> MSKVMKPSNGKGSRKSSKAATPDTKNFFHAKKKDPVNQDKANNASQITPTVPHSHPSDMVIPDHLAELIPELYSFQQLVDSEKRLDHFIHLRNLHMKRMVAQWERSKLSQEFLYPHLNFPNVKFLRIFISNVSENQPWQMDTNNEADLMALENATWTMRIEGRLLDNVQANDPAREKFSSFIESIVVDFKNKENDNVPSTKFNAAPEENATEGPSDKKLNLNLPLQFSLPNGDNSTTTNTDQNNATMGEETAKKDMSSTTPKLESVKWQYDPNNPVDFDGLDIKRVGSENVECTISILRKSSPEEPFMSYSPQLTAIIGLKSGTSHDAIFSIYKYIHLNELLTNDESAFENLMGNRNNHNSNTSTSKMLDAASSQVSIVKLDTQLITLLPSSLKESSPDTMKLTDLLSLINSTHLLPLQPIEIDYTVRVDKASTYGELVLDIEVPDVNALKFNNTQRESQIGAAELNENARELEQIKPKIALQDKEITSVLSNLHESNKRYRFFKKISEDPVKALNECIASTSNALKVLSGDEGYNEDMVRRANFYKENEAMLRENIEVILSNGRM;>MENTLGEGSTVNASVDVDQHGNDNNSDSNANAAVAGVANTDTAGEESQQQDESLKDEATVPNTRDAESEAITVTAKQQPTMQANKLDSQETPSTEESRAQNVFGQDNEDSDNLFGETESSVSNNEANTPSIPTNPVDNENNKPAIKEDSTIQDSNGDVKNMEDVKIQKEEEPENNTVIEGVKEESQPDENTKEMDEVEEDDEDDDQPMISPDNSIFGDTKSESKQLGNTSSVANTPSEIPDAHKAEQEDIIEKTESVDKKVDSGEERNEQEREIMNDHSKSANPKKTTITRVEPETFEIPQAHEIVIPSYSKWFNLEKIHSIEVQSLPEFFTNRIPSKTPEVYMRYRNFMVNSYRLNPNEYFSVTTARRNVSGDAAALFRLHKFLTKWGLINYQVDSKLLPKNIEPPLTSQYSTRHDAPRGLFPFESYKPSVQLPDMAKLKKMMNTSDSESTLYKYLKESKRKYDEITHPPSTTDDENGDKNDNGGKMNNEVSTSTSMTGDANLLEEGETSRPLKKVKILEQIDENWSKEDLQKLLKGIQEFGADWYKVAKNVGNKSPEQCILRFLQLPIEDKFLYGDGNGKGDNDNGLGPLKYAPHLPFSKSENPVLSTIAFLVGLVNPKTVQSMTQRAIQSAESIKSQKEEISDQKPIEHIKEGSEIAISSLGYRSHIFATNEERQMNFLTNELIRLQMEKLDAKLNHLKKLEKFMELERKTLERQQENLLIQRLNFNQNSSKIVNVLSKCLNLISDSNINNSSVAEKEEIRSQIDHFKSMLSKPETLSIGKNPFNKPNIETGENHNGQSISNENDVKPISIEAPQFYRYWSA[2x];> MGVIKKKRSHHGKASRQQYYSGVQVGGVGSMGAINNNIPSLTSFAEENNYQYGYSGSSAGMNGRSLTYAQQQLNKQRQDFERVRLRPEQLSNIIHDESDTISFRSNLLKNFISSNDAFNMLSLTTVPCDRIEKSRLFSEKTIRYLMQKQHEMKTQAAELQEKPLTPLKYTKLIAAAEDGSRSTKDMIDAVFEQDSHLRYQPDGVVVHRDDPALVGKLRGDLREAPADYWTHAYRDVLAQYHEAKERIRQKEVTAGEAQDEASLQQQQQQDLQQQQQVVTTVASQSPHATATEKEPVPAVVDDPLENMFGDYSNEPFNTNFDDEFGDLDAVFF;> MLGEDEGNTVLEKGNNPSVKQGEVGAVFIVPKILIREHERVILKQILQILDQDELVQPPLDKFPYKKLELPKYIDELKTRDATNTSYKMIQLDAYGEKKVGSNGELFGGRHYLFNTFTFTAHMGVLLVLLQDVIKVLYQSNATHDEDEFIVQHDQILVMETSEEQTKFLAKNGVIPEESKGSFKYITARSAFVEFGASVIAGGQRIVDDYWESLAKKQNLSSHQRVFKLSTNLISKISLLRPSFQNNRISNANEISANTNNTCTISTSKFESQYPIVTEQPSAEIREAYIENFAKGEHISAIVPGQSISGTLELSAQFRVPRYHSKNSFQQALQMKAMDIPIGRHEELLAQYESQAPDGSASISLPNHIPSVNPSNKPIKRMLSSILDINVSSSKNKKSEENEMIKPMNKGQHKNNTSLNINGWKFESLPLKSAENSGKQQYYRGLPLYEKNTLLERLKQLTPNEIKELEHLHDAVFVNTGLQNVRKVRTKKWKKYWQYKAGIPIGLKRSQLDEFKNKYLKDVLAQTSVTTNFNEITNTDETITTKRVPNPNFLGNCNIKDFKPPYIYSHVNKVPQNVAGDKTAVKLDTEVKNTNANPVVATDPVAAKPDNLANFSNEVAMNN;> MNNQPQGTNSVPNSIGNIFSNIGTPSFNMAQIPQQLYQSLTPQQLQMIQQRHQQLLRSRLQQQQQQQQQTSPPPQTHQSPPPPPQQSQPIANQSATSTPPPPPAPHNLHPQIGQVPLAPAPINLPPQIAQLPLATQQQVLNKLRQQAIAKNNPQVVNAITVAQQQVQRQIEQQKGQQTAQTQLEQQRQLLVQQQQQQQLRNQIQRQQQQQFRHHVQIQQQQQKQQQQQQQHQQQQQQQQQQQQQQQQQQQQQQQQQQQQQQQQQQQQQGQIPQSQQVPQVRSMSGQPPTNVQPTIGQLPQLPKLNLPKYQTIQYDPPETKLPYPTYWSDKKADTDTLLYEQIIQRDKINKYSLIRETNGYDPFSIYGFSNKEYISRLWHTLKYYQDLKNTRMKSITSTSQKIPSASIWGNGYSGYGNGITNTTTRVIPQVEVGNRKHYLEDKLKVYKQAMNETSEQLVPIRLEFDQDRDRFFLRDTLLWNKNDKLIKIEDFVDDMLRDYRFEDATREQHIDTICQSIQEQIQEFQGNPYIELNQDRLGGDDLRIRIKLDIVVGQNQLIDQFEWDISNSDNCPEEFAESMCQELELPGEFVTAIAHSIREQVHMYHKSLALLGYNFDGSAIEDDDIRSRMLPTITLDDVYRPAAESKIFTPNLLQISAAELERLDKDKDRDTRRKRRQGRSNRRGMLALSGTSASNTSMNGVHNTVAAGNASSLPPGEILLPDIADIPRTFRTPVPSTLMPGGVDVGPSVESYELRNTTTYKSRPDRPKPVSPPCYIIDHIPGHSLLLSIKLPGKVNTKEEFAAAPNDTSSGTNAMLPSPESLKTKLNSNIRAGVTIPSIPNPIANHTVTNSPNPTLQPVIPGGAASKSVPTPSLPIAPPVAPHDSEATLLTNSNNGSSNNNTQNT;> MNIPQRQFSNEEVNRCYLRWQHLRNEHGMNAPSVPEFIYLTKVLQFAAKQRQELQMQRQQQGISGSQQNIVPNSSDQAELPNNASSHISASASPHLAPNMQLNGNETFSTSAHQSPIMQTQMPLNSNGGNNMLPQRQSSVGSLNATNFSPTPANNGENAAEKPDNSNHNNLNLNNSELQPQNRSLQEHNIQDSNVMPGSQINSPMPQQAQMQQAQFQAQQAQQAQQAQQAQQAQARLQQGRRLPMTMFTAEQSELLKAQITSLKCLVNRKPIPFEFQAVIQKSINHPPDFKRMLLSLSEFARRRQPTDQNNQSNLNGGNNTQQPGTNSHYNNTNTDNVSGLTRNAPLDSKDENFASVSPAGPSSVHNAKNGTLDKNSQTVSGTPITQTESKKEENETISNVAKTAPNSNKTHTEQNNPPKPQKPVPLNVLQDQYKEGIKVVDIDDPDMMVDSFTMPNISHSNIDYQTLLANSDHAKFTIEPGVLPVGIDTHTATDIYQTLIALNLDTTVNDCLDKLLNDECTESTRENALYDYYALQLLPLQKAVRGHVLQFEWHQNSLLTNTHPNFLSKIRNINVQDALLTNQLYKNHELLKLERKKTEAVARLKSMNKSAINQYNRRQDKKNKRLKFGHRLIATHTNLERDEQKRAEKKAKERLQALKANDEEAYIKLLDQTKDTRITHLLRQTNAFLDSLTRAVKDQQKYTKEMIDSHIKEASEEVDDLSMVPKMKDEEYDDDDDNSNVDYYNVAHRIKEDIKKQPSILVGGTLKDYQIKGLQWMVSLFNNHLNGILADEMGLGKTIQTISLLTYLYEMKNIRGPYLVIVPLSTLSNWSSEFAKWAPTLRTISFKGSPNERKAKQAKIRAGEFDVVLTTFEYIIKERALLSKVKWVHMIIDEGHRMKNAQSKLSLTLNTHYHADYRLILTGTPLQNNLPELWALLNFVLPKIFNSVKSFDEWFNTPFANTGGQDKIELSEEETLLVIRRLHKVLRPFLLRRLKKDVEKELPDKVEKVVKCKMSALQQIMYQQMLKYRRLFIGDQNNKKMVGLRGFNNQIMQLKKICNHPFVFEEVEDQINPTRETNDDIWRVAGKFELLDRILPKLKATGHRVLIFFQMTQIMDIMEDFLRYINIKYLRLDGHTKSDERSELLRLFNAPDSEYLCFILSTRAGGLGLNLQTADTVIIFDTDWNPHQDLQAQDRAHRIGQKNEVRILRLITTNSVEEVILERAYKKLDIDGKVIQAGKFDNKSTSEEQEALLRSLLDAEEERRKKRESGVEEEEELKDSEINEILARNDEEMAVLTRMDEDRSKKEEELGVKSRLLEKSELPDIYSRDIGAELKREESESAAVYNGRGARERKTATYNDNMSEEQWLRQFEVSDDEKNDKQARKQRTKKEDKSEAIDGNGEIKGENIDADNDGPRINNISAEDRADTDLAMNDDDFLSKKRKAGRPRGRPKKVKLEGSENSEPPALESSPVTGDNSPSEDFMDIPKPRTAGKTSVKSARTSTRGRGRGRGRGRGRGRGRGRPPKARNGLDYVRTPAAATSPIDIREKVAKQALDLYHFALNYENEAGRKLSDIFLSKPSKALYPDYYMIIKYPVAFDNINTHIETLAYNSLKETLQDFH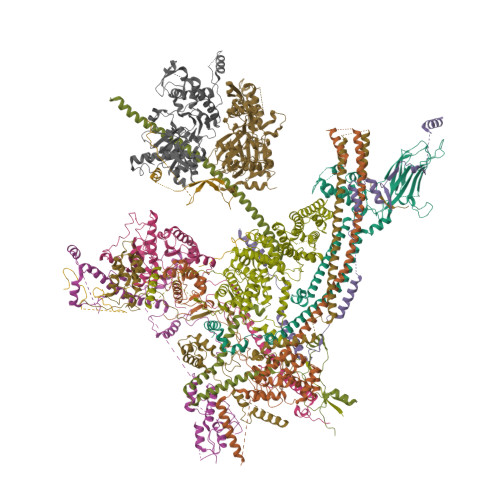LIFSNARIYNTEGSVVYEDSLELEKVVTKKYCEIMGDNSQLDFTEFDEQYGTRPLVLPPVVTSSVAESFTDEADSSMTEASV;> MDFFNLNNNNNNNNTTTTTTTTNNNNTNNNNTNNNNNPANNTNNNNSTGHSSNTNNNTNNNNTNTGASGVDDFQNFFDPKPFDQNLDSNNNNSNSNNNDNNNSNTVASSTNFTSPTAVVNNAAPANVTGGKAANFIQNQSPQFNSPYDSNNSNTNLNSLSPQAILAKNSIIDSSNLPLQAQQQLYGGNNNNNSTGIANDNVITPHFITNVQSISQNSSSSTPNTNSNSTPNANQQFLPFNNSASNNGNLTSNQLISNYAASNSMDRSSSASNEFVPNTSDNNNNSNNHNMRNNSNNKTSNNNNVTAVPAATPANTNNSTSNANTVFSERAAMFAALQQKQQQRFQALQQQQQQQQNQQQQNQQPQQQQQQQQNPKFLQSQRQQQQRSILQSLNPALQEKISTELNNKQYELFMKSLIENCKKRNMPLQSIPEIGNRKINLFYLYMLVQKFGGADQVTRTQQWSMVAQRLQISDYQQLESIYFRILLPYERHMISQEGIKETQAKRIFLQQFLQELLKKVQQQQQAAALANANNNINSASSAPTPAAPGASVPATAAPGTEAGIVPVSANTPKSLNSNININVNNNNIGQQQVKKPRKQRVKKKTKKELELERKEREDFQKRQQKLLEDQQRQQKLLLETKLRQQYEIELKKLPKVYKRSIVRNYKPLINRLKHYNGYDINYISKIGEKIDSNKPIFLFAPELGAINLHALSMSLQSKNLGEINTALNTLLVTSADSNLKISLVKYPELLDSLAILGMNLLSNLSQNVVPYHRNTSDYYYEDAGSNQYYVTQHDKMVDKIFEKVNNNATLTPNDSNDEKVTILVDSLTGNQLPTPTPTEMEPDLDTECFISMQSTSPAVKQWDLLPEPIRFLPNQFPLKIHRTPYLTSLKKIKDEIDDPFTKINTRGAEDPKVLINDQLSTISMILRNISFSDNNSRIMSRNFYLKRFISDLLWLVLIHPENFTCNRKILNFKKDLVIVLSNISHLLEIASSIDCLLILILVISFGQPKLNPMASSSSFGSESLTFNEFQLQWGKYQTFGVDILAKLFSLEKPNLNYFKSILLNKNTGNNLYDRNSNNNHKDKKLLRRLLNLYNDNNKNNNNRHNLLNDVVSFLFSAIPLQQVLSQSADPSLLIDQFSPVISQSLTSILVIVQKILPLSNEVFEISENNSDSNSNNNGNKDSSFNFNKNLPFVWLSSEENIGSGLLKLSEIILNINNSTSKNTLLQQQNYSKVLLPSINISCVQLIKCLVEKSICFENCLNNDPEILKKIASIPNLFPTDLEIFQLFTNPSVDIQIINQYQLLYNLKNDILTNLE;> MDPQTLITKANKVSYYGNPTSKESWRYDWYQPSKVSSNVQQPQQQLGDMENNLEKYPFRYKTWLRNQEDEKNLQRESCEDILDLKEFDRRILKKSLMTSHTKGDTSKATGAPSANQGDEALSVDDIRGAVGNSEAIPGLSAGVNNDNTKESKDVKMN;> MTLNRKCVVIHNGSHRTVAGFSNVELPQCIIPSSYIKRTDEGGEAEFIFGTYNMIDAAAEKRNGDEVYTLVDSQGLPYNWDALEMQWRYLYDTQLKVSPEELPLVITMPATNGKPDMAILERYYELAFDKLNVPVFQIVIEPLAIALSMGKSSAFVIDIGASGCNVTPIIDGIVVKNAVVRSKFGGDFLDFQVHERLAPLIKEENDMENMADEQKRSTDVWYEASTWIQQFKSTMLQVSEKDLFELERYYKEQADIYAKQQEQLKQMDQQLQYTALTGSPNNPLVQKKNFLFKPLNKTLTLDLKECYQFAEYLFKPQLISDKFSPEDGLGPLMAKSVKKAGASINSMKANTSTNPNGLGTSHINTNVGDNNSTASSSNISPEQVYSLLLTNVIITGSTSLIEGMEQRIIKELSIRFPQYKLTTFANQVMMDRKIQGWLGALTMANLPSWSLGKWYSKEDYETLKRDRKQSQATNATN;> MAPFRQDSILIIYPRSQTTLVQFGLNEETFTVPELEIPTQIYRTTRQDGSYTYHSTNKDNKAELIKPIQNGEIIDISAFTQFLRLIFVSILSDRANKNQDAFEAELSNIPLLLITHHSWSQSDLEIITQYVFESLEINNLIQLPASLAATYSMISLQNCCIIDVGTHHTDIIPIVDYAQLDHLVSSIPMGGQSINDSLKKLLPQWDDDQIESLKKSPIFEVLSDDAKKLSSFDFGNENEDEDEGTLNVAEIITSGRDTREVLEERERGQKVKNVKNSDLEFNTFWDEKGNEIKVGKQRFQGCNNLIKNISNRVGLTLDNIDDINKAKAVWENIIIVGGTTSISGFKEALLGQLLKDHLIIEPEEEKSKREEEAKSVLPAATKKKSKFMTNSTAFVPTIEYVQCPTVIKLAKYPDYFPEWKKSGYSEIIFLGAQIVSKQIFTHPKDTFYITREKYNMKGPAALWDVQF> SRCDMYLTMDL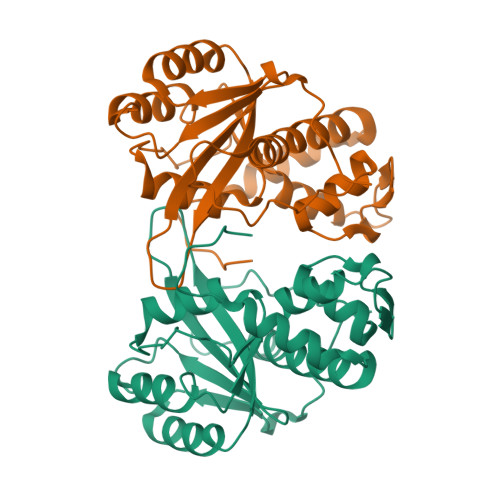PDECLIIVNKADEFDRMLYHLQQECVIYLASEWMQSVCGDNQLCVLQIATGHNVYLIDCLARESLRSEHWRLLGANIFNNVNIRKVGFSMVSDLSVLQRSLPLQLRLQMPHHYLDLRNLWLELKKQRFGVELPFGNVNRAGDALTDLSLACLGKKLNKSNQCSNWANRPLRREQILYAAIDARCLMLIYNTLIERVSFIQAVIEKSIASNNFLRRGAHVK>ETGDQRFGDLVFRQLAPNVWQHTSYLDMPGFGAVASNGLIVRDGGRVLVVDTAWTDDQTAQILNWIKQEINLPVALAVVTHAHQDKMGGMDALHAAGIATYANALSNQLAPQEGMVAAQHSLTFAANGWVEPATAPNFGPLKVFYPGPGHTSDNITVGIDGTDIAFGGCLIRDSKAKS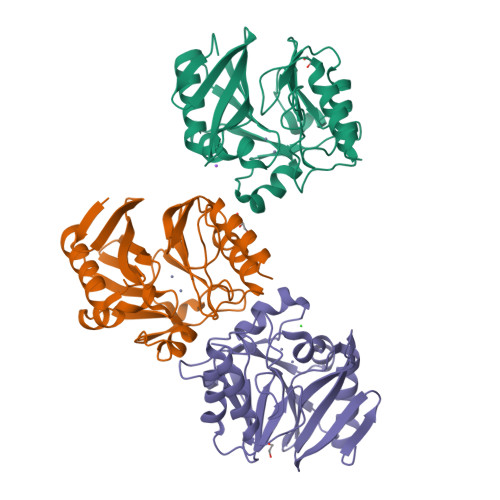LAQLGDADTEHYAASARAFGAAFPKASMIVMSHSAPDSRAAITHTARMADKLR[4x]>[2x]MVAPESIVLRVARLDELEQVREILHRIYYPEEGITISYVHGKSHTLDDERFSLSFVEQGTVVVAEDSAAKKFIGVSIAGPIQPGDPDAMVEEAA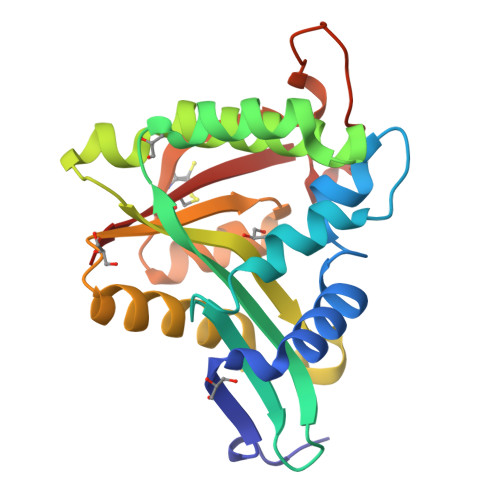TTETKKWGDILKLLALLERTADVCGRYGLEKAYHVHILAVDPTYRGHSLGQRLLQFQMDLSKKLGFKAISGDFTSVFSVKLAEKLGMECISQLALGDYRDEKGEKLFEPLDVHQVIKTCVKLL>[8x]GGGGTTTTG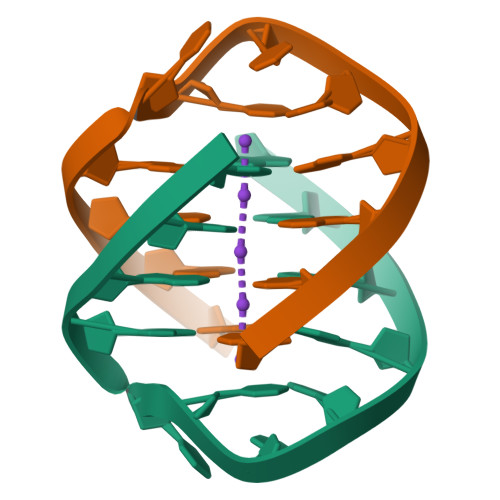GGG(S)-2-(3-(6-amino-9H-purin-9-yl)propoxy)-3-phosphonopropanoic acid | C11 H16 N5 O6 P | 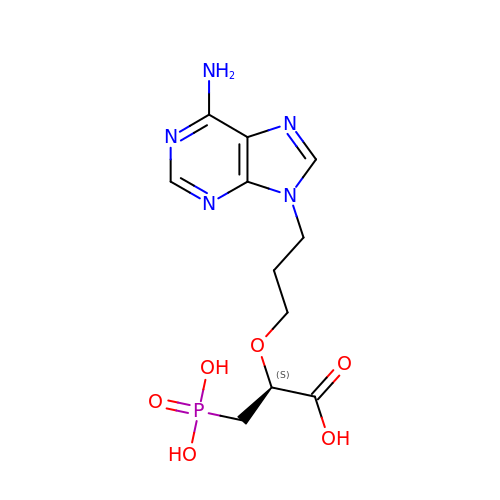XOIURUPPHSOSSY-SSDOTTSWSA-N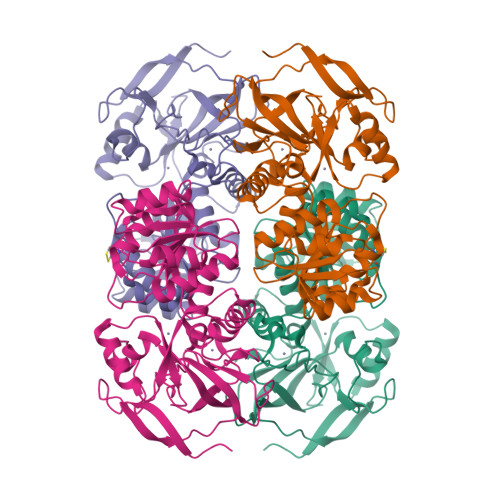>[4x]SIPETQKGVIFYESHGKLEYKDIPVPKPKANELLINVKYSGVCHTDLHAWHGDWPLPVKLPLVGGHEGAGVVVGMGENVKGWKIGDYAGIKWLNGSCMACEYCELGNESNCPHADLSGYTHDGSFQQYATADAVQAAHIPQGTDLAQVAPILCAGITVYKALKSANLMAGHWVAISGAAGGLGSLAVQYAKAMGYRVLGIDGGEGKEELFRSIGGEVFIDFTKEKDIVGAVLKATDGGAHGVINVSVSEAAIEASTRYVRANGTTVLVGMPAGAKCCSDVFNQVVKSISIVGSYVGNRADTREALDFFARGLVKSPIKVVGLSTLPEIYEKMEKGQIVGRYVVDTSK> MADPMAGLELLSDQGYRVDGRRAGEL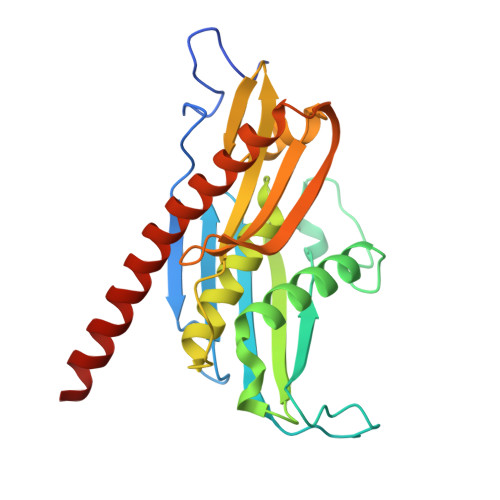RKIQARMGVFAQADGSAYIEQGNTKALAVVYGPHEIRGSRARALPDRALVNCQYSSATFSTGERKRRPHGDRKSCEMGLQLRQTFEAAILTQLHPRSQIDIYVQVLQADGGTYAACVNAATLAVLDAGIPMRDFVCACSAGFVDGTALADLSHVEEAAGGPQLALALLPASGQIALLEMDARLHEDHLERVLEAAAQAARDVHTLLDRVVRQHVREASILLGD The major regulator of virulence factors in L. monocytogenes is the transcription activator PrfA, a member of the Crp/Fnr family of regulators. PrfAWT is a homodimer in which each monomer consists of an N-terminal domain (residues 1 to 108) and a C-terminal DNA-binding domain (residues 138 to 237) linked by a long α-helix (αC, residues 109 to 137). Two α-helices in the C-terminal domain, αE (residues 170 to 178) and αF (residues 183 to 197), constitute the two helices of the typical HTH motif present in many prokaryotic transcription factors. Glutathione binding stabilizes the DNA-binding helix-turn-helix (HTH) motif in a conformation compatible with DNA-binding, thereby allowing expression of PrfA-regulated virulence factors.

In addition, we found three new PrfA mutants in the remaining three strains—Leu to His substitution at residue 140 (PrfAL140H), Ala to Gly substitution at residue 218 (PrfAA218G), and Ala to Val substitution at residue 94 (PrfAA94V). To gain a deeper understanding of the PrfA* mutant proteins, the crystal structures of purified PrfAL140H, PrfAL140F, and PrfAA218G were determined as individual proteins and in complex with the PrfA hly promoter DNA. Here, we show that all the PrfA* proteins identified in our screen had higher binding affinities to hly, actA, and hpt promoter sequences than the PrfAWT protein. The previously identified PrfAG145S protein showed the lowest equilibrium binding constant, i.e., strongest binding of all the mutants, followed by the PrfAA218G, PrfAL140H, and PrfAL140F proteins, respectively. However, when PrfA is bound to promoter DNA, both monomers are almost identical to each other in all of our PrfA mutants.

>GAMNAQAEEFKKYLETNGIKPKQFHKKELIFNQWDPQEYCIFLYDGITKLTSISENGTIMNLQYYKGAFVIMSGFIDTETSVGYYNLEVISEQATAYVIKINELKELLSKNLTHFFYVFQTLQKQVSYSLAKFNDFSINGKHGSICGQLLILTYVYGKETPDGIKITLDNLTMQELGYSSGIAHSSAVSRIISKLKQEKVIVYKNSCFYVQNLDYLKRYAPKLDEWFYLACPATWGKLN[2x]> RVDVSLPGASLFSGGLHPITLMERELVEIFRALGYQAVEGPEVESEFFNFDALNIPEHHPARDMWDTFWLTGEGFRLEGPLGEEVEGRLLLRTHTSPMQVRYMVAHTPPFRIVVPGRVFRFEQTDATHEAVFHQLEGLVVGEGIAMAHLKGAIYELAQALFGPDSKVRFQPVYFPFVEPGAQFAVWWPEGGKWLELGGAGMVHPKVFQAVDAYRERLGLPP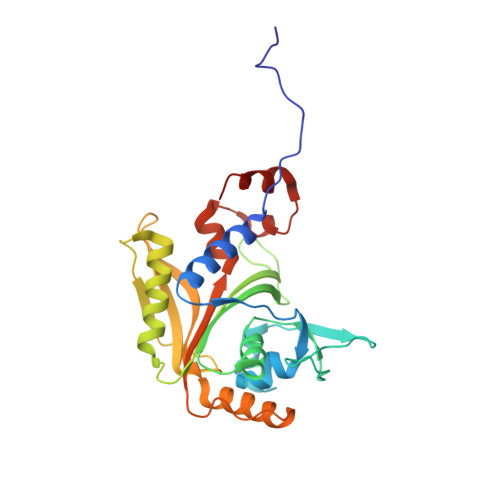AYRGVTGFAFGLGVERLAMLRYGIPDIRYFFGGRLKFLEQFKGVL>[2x]ENEIERPEDMRVRTLANK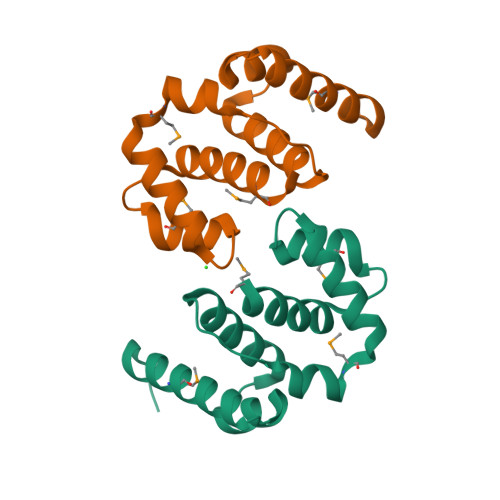SKMKVSIVQQIDRKVALDDIAVSHGLDFPELLSEVETIVYSGTRINIDYFINEVMDEDHLEDIFEYFKESTTDSLEEAMQELGKDYSEEEIRLVRIKFLSEMAN2-METHYLPROPANAMIDE | C4 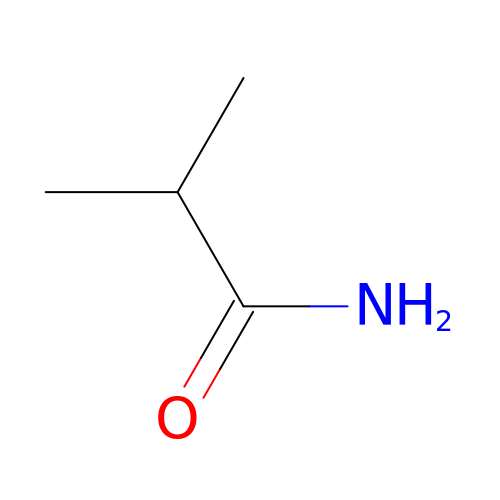H9 N O | WFKAJVHLWXSISD-UHFFFAOYSA-N>[2x]HMSFLTEEEQEAIMKVLQRDAALKRAEEERGSGSGSGMSDGDYDYLIKFLALGDSGVGKTSVLYQYTDGKFNSKFITTVGIDFREKRVVYRASGPDGATGRGQRIHLQLWDTAGLERFRSLTTAFFRDAMGFLLLFDLTNEQSFLNVRNWISQLQMHAYCENPDIVLCGNKSDLEDQRVVKEEEAIALAEKYGIPYFETSAANGTNISQAIEMLLDLIMKRMERSVDKS

Rab27A and Rab27B are secretory Rabs with well-characterised roles in transport and docking of secretory vesicles (exosomes) at the plasma membrane. Rab27A promotes the growth and invasion of multiple cancer types such as breast, lung and pancreatic, by enhancing secretion of chemokines, metalloproteases and exosomes. Reported co-crystal structures show that several effectors of Rab27A interact with the Rab27A SF4 pocket (‘WF-binding pocket’) via a conserved tryptophan–phenylalanine (WF) dipeptide motif. To obtain structural insight into the ligandability of this pocket, a novel construct was designed fusing Rab27A to part of an effector protein (fRab27A), allowing crystallisation of Rab27A in high throughput.

Covalent ligands are increasingly used to target challenging proteins. fRab27A contains two cysteine residues (C123 and C188) in close proximity to the WF-binding pocket, which are mutated to serine in crystal structures. Sequence alignment of Rab27A and Rab27B against the Rab family demonstrated that these two cysteine residues are unique to Rab27 among other family members (Fig. 1C and S4†), suggesting that cysteine-reactive covalent fragments targeting the WF binding site may offer a means to ligand Rab27 selectively over other Rabs. Compounds A01 and B01 were confirmed as hits against fRab27A-C188 and fRab27A-C123, respectively. Hit fragment A01 preferentially reacted with fRab27A-C188, whereas fragment B01 was found to react with both fRab27A-C123 and fRab27A-C188 with significant rate enhancement over GSH. Residues K11 and D91 were located in close proximity to the methyl ether moiety, suggesting a route to build further polar contacts in analogues of A01. The structure of B01 bound to fRab27A-C123 demonstrated similar hydrophobic interactions with M93 and M185 (see Fig. S7B† for the density map). However, in contrast to the fRab27A-C188-A01 structures, in which the SF4 pocket is largely unperturbed by C188 modification, and the Rab27A-Slp2a complex, C123 modification by B01 caused the side chain of Y122 to adopt an alternate conformation, opening up an enlarged cavity in the pocket. Interestingly, molecular dynamic simulations on Rab27A (PDB: 3 BC1, chain A) suggested that the Y122 sidechain has three main rotamers with the rotamer trapped by the fRab27A-C123-B01 complex as the preferred conformation (Fig. S8A†). The B01 fragment was also positioned with potential fragment growth vectors to form polar interactions with K11 and D91.>[2x]GSARPSSSMADFRKFFAKAKHIVIISGAGVSAESGVPTFRGAGGYWRKWQAQDLATPLAFAHNPSRVWEFYHYRREVMGSKEPNAGHRAIAECETRLGKQGRRVVVITQNIDELHRKAGTKNLLEIHGSLFKTRCTSCGVVAENYKSP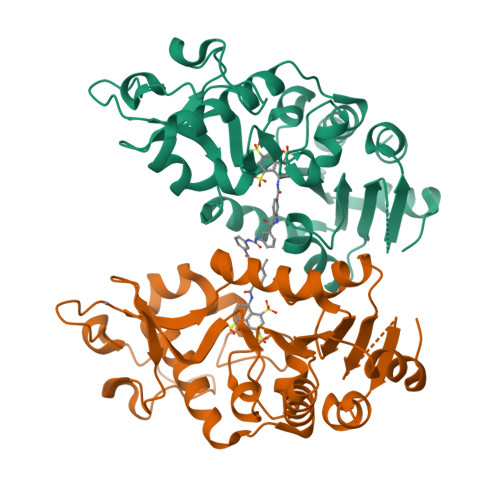ICPALSGKGAPEPGTQDASIPVEKLPRCEEAGCGGLLRPHVVWFGENLDPAILEEVDRELAHCDLCLVVGTSSVVYPAAMFAPQVAARGVPVAEFNTETTPATNRFRFHFQGPCGTTLPEALA> SQIGETLENIRSIEKLIQNIMRIARETN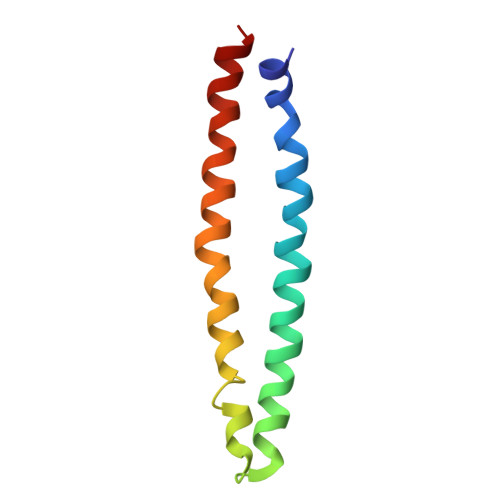ILALNATIEAARAGEAGKGFMIVANEVQNLSNETNEVTKQIVEKAREILESSQRSLE Proteinaceous brain inclusions containing the transactive response DNA-binding protein of 43 kDa (TDP-43) are a pathological hallmark of amyotrophic lateral sclerosis (ALS) and frontotemporal lobar degeneration (FTLD). TDP-43 consists of an N-terminal domain, two RNA recognition motifs, and a C-terminal low-complexity domain (LCD) that maps to residues ~267–414 and is rich in Gln/Asn and Gly residues. Furthermore, recent reports indicate that these aggregates can self-propagate by the prion-like mechanism. Consistent with these findings, polypeptides corresponding to TDP-43 LCD or its fragments have been shown to form amyloid fibrils in vitro.

Here, we report the cryo-EM structure of amyloid formed from the entire TDP-43 low complexity domain in vitro at pH 4. Each twisted fibril consists of a single left-handed protofilament in which subunits stack along the fibril axis with a helical rise of 4.73 Å and a helical twist of −1.66°. A near-atomic-resolution structural model could be unambiguously built for the fibril core, which maps to residues 276–414 of TDP-43. The C-terminal region (residues 344–414, strands β9–β14) is characterized by a small proportion of hydrophobic amino acids. Relatively long β-strands pack mostly via polar interfaces and many residues within strands β9, β10, β11, and β13 are engaged in steric–zipper interactions. By contrast, the N-terminal region of LCD (residues 276–343, strands β1–β8) is rich in hydrophobic amino acids and contains mostly short β-strands that are not involved in steric–zipper interactions. Instead, strands and turns pack against each other in all directions, allowing non-polar side chains to be tightly packed and buried, with a hydrophobic interface between the 311–318 and 336–341 segments. The non-planar backbone conformation of TDP-43 LCD subunits (which is not unusual among amyloids) results in rugged surfaces of fibril ends with well-defined “ridges” and “grooves”. Mapping the pathogenic mutations on the structure of wild-type TDP-43 LCD fibrils revealed that ~50% of them are not compatible with this structure due to severe steric clashes within tightly packed segments of the protein, introduction of charges into the dehydrated fibril interior, or both.

>[5x]NRQLERSGRFGGNPGGFGNQGGFGNSRGGGAGLGNNQGSNMGGGMNFGAFSINPAMMAAAQAALQSSWGMMGMLASQQNQSGPSGNNQNQGNMQREPNQAFGSGNNSYSGSNSGAAIGWGSASNAGSGSGFNGGFGSSMDSKSSGWGM> SISQQTVWNQMATVRTPLNFDSSKQSFCQFSVDLLGGGISVDKTGDWITLVQNSPISNLLRVAAWKKGCLMVKVVMSGNAAVKRSDWASLVQVFLTNSNSTEHFDACRWTKSEPHSWELIFPIEVCGPNNGFEMWSSEWANQTSWHLSFLVDNPKQSTTFDVLLGISQNFEIAGNTLMPAFSVPQ;> METNLFKLSLDDVETPKGSMLDLKISQSKIALPKNTVGGTILRSDLLANFLTEGNFRASVDLQRTHRIKGMIKMVATVGIPENTGIALACAMNSSIRGRASSDIYTICSQDCELWNPACTKAMTMSFNPNPCSDAWSLEFLKRTGFHCDIICVTGWTATPMQDVQVTIDWFISSQECV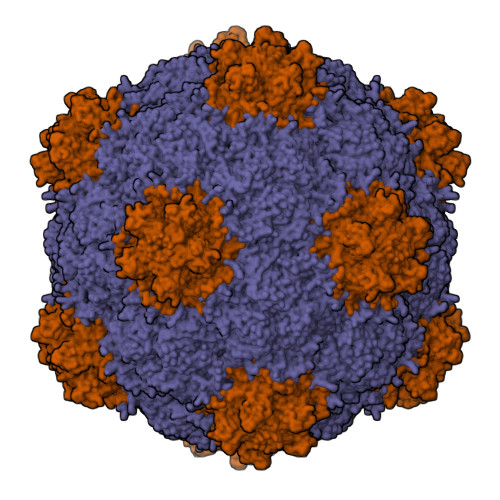PRTYCVLNPQNPFVLNRWMGKLTFPQGTSRSVKRMPLSIGGGAGAKSAILMNMPNAVLSMWRYFVGDLVFEVSKMTSPYIKCTVSFFIAFGNLADDTINFEAFPHKLVQFGEIQEKVVLKFSQEEFLTAWSTQVRPATTLLADGCPYLYAMVHDSSVSTIPGDFVIGVKLTIIENMCAYGLNPGISGSRLLG> GP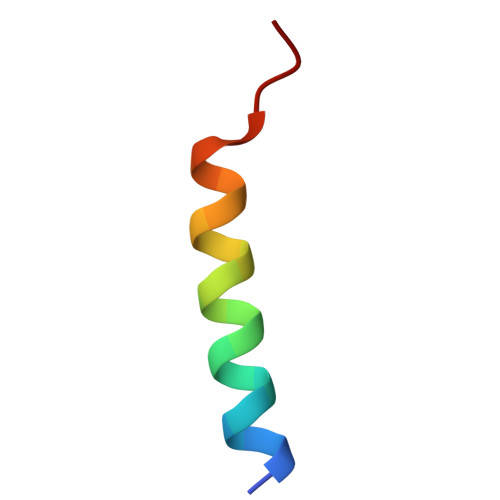MEEQREILEQLKKTLQMLTVY>GPLGSMKTVFSPLHS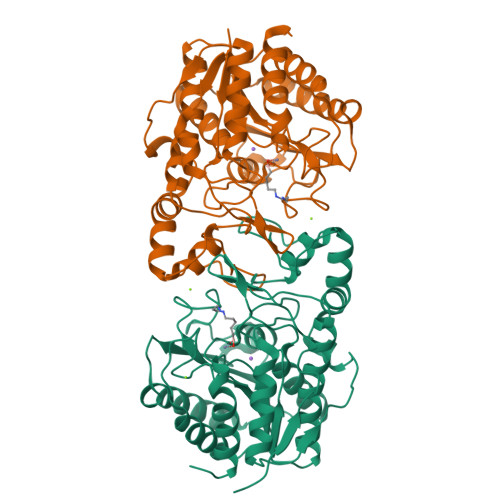RRHVKTELDGGLLIEPHEKPSRAETILARVKDQALGEILEPEEFGLGPVKRVHTADYVSFLETCWDEWVAAGKRGEAIPTFWVGRGMRARLPKDIDGRLGYYSLGADTSISDGTWEAARASANVALTAQKLVAEGERAAFALCRPPGHHAHADVFGGYCFFNNAAIAAQAFRDQGYGKVAVLDVDFHHGNGTQAIFYDRSDVLTISLHGDPDLVFPHFLGFEDETGEGDGEAYNLNIVFPPDTPFSIWSQGLEKACERIRTFAPDALVVALGVDTFEEDPISFFKLTSGDYLKLGKRLEQLGLPTVFTMEGGYDVDAIGVNAVNVMQGFEGKS[4x]4-(bromomethyl)benzoic acid | C8 H7 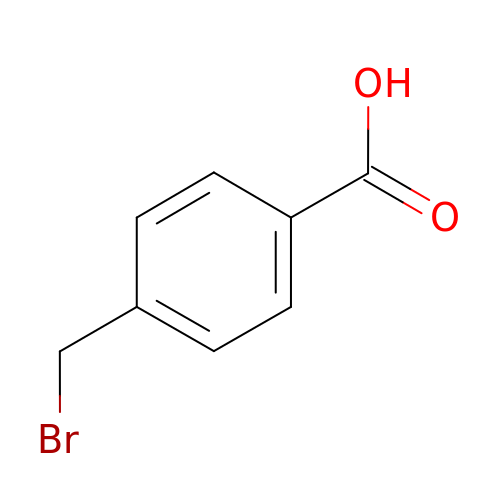Br O2 | CQQSQBRPAJSTFB-UHFFFAOYSA-N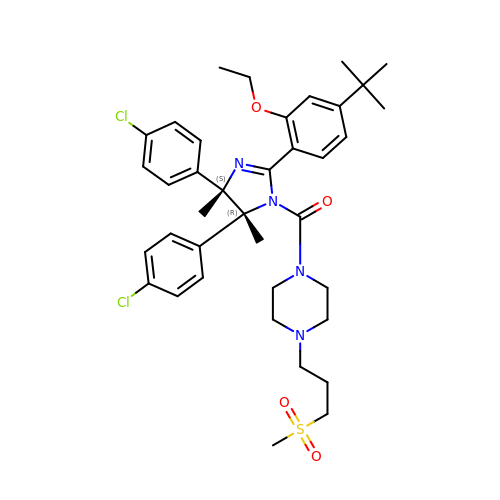[(4S,5R)-2-(4-tert-butyl-2-ethoxyphenyl)-4,5-bis(4-chlorophenyl)-4,5-dimethyl-4,5-dihydro-1H-imidazol-1-yl]{4-[3-(methylsulfonyl)propyl]piperazin-1-yl}methanone | C38 H48 Cl2 N4 O4 S | QBGKPEROWUKSBK-QPPIDDCLSA-N>QAKILEADAEILKAYAKILEAHAEILKAQ[1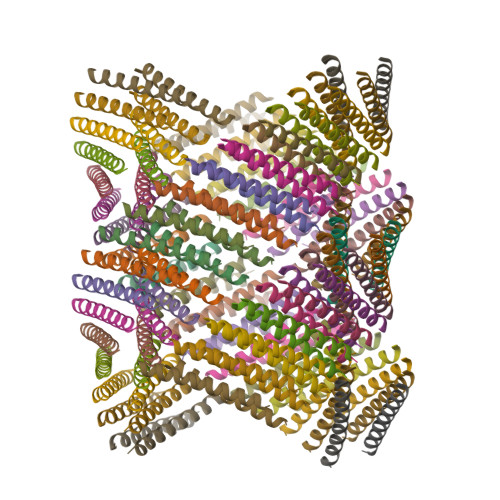06x]>[4x]MAKEFGIPAAVAGTVLNVVEAGGWVTTIVSILTAVGSGGLSLLAAAGRESIKA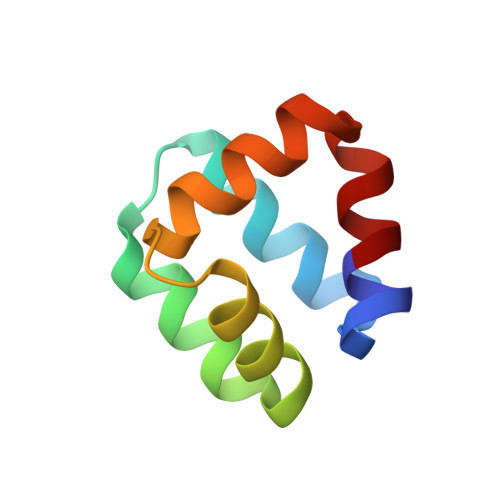YLKKEIKKKGKRAVIAW> SNADSSRRQYQEKYKQVEQYMSFHKLPADFRQKIHDYYEHRYQGKMFDEDSILGELNGPLREEIVNFNCRKLVASMPLFANADPNFVTAMLTKLKFEVFQPGDYIIRE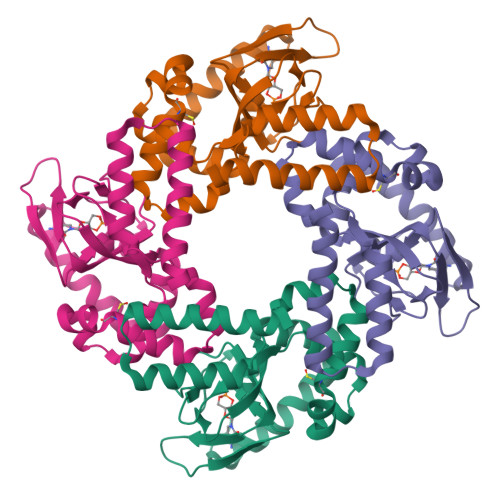GTIGKKMYFIQHGVVSVLTKGNKEMKLSDGSYFGEICLLTRGRRTASVRADTYCRLYSLSVDNFNEVLEEYPMMRRAFETVAIDRLDRIGKKNSIL>GSHGMVSVSEIRKAQRAEGPATILAIGTANPANCVEQSTYPDFYFKITNSEHKTELKEKFQRMCDKSMIKRRYMYLTEEILKENPNVCEYMAPSLDARQAMLAMEVPRLGKEAAVKAIKEWGQPKSKITHLIVCSTTTPDLPGADYQLTKLLGLRPYVKRVGVFQHGCFAGGTVLRLAKDLAENNKGARVLVVCSEVTAVTFRGPSDTHLDSLVGQALFGDGAAALIVGSDPVPEIEKPIFEMVWTAQTIAPDSEGAIDGHLREAGLTFHLKGAVPDIVSKNITKALVEAFEPLGISDYNSIFWIAHPGGPAILDQV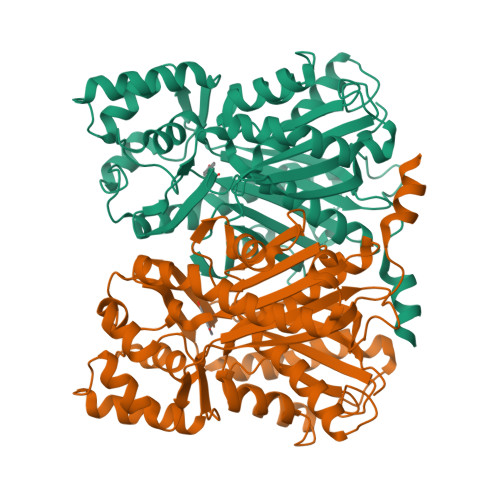EQKLALKPEKMNATREVLSEYGNMSSACVLFILDEMRKKSTQNGLKTTGEGLEWGVLFGFGPGLTIETVVLRSVAI[4x]> MLEQPYLDLAKKVLDEGHFKPDRTHTGTYSIFGHQMRFDLSKGFPLLTTKKVP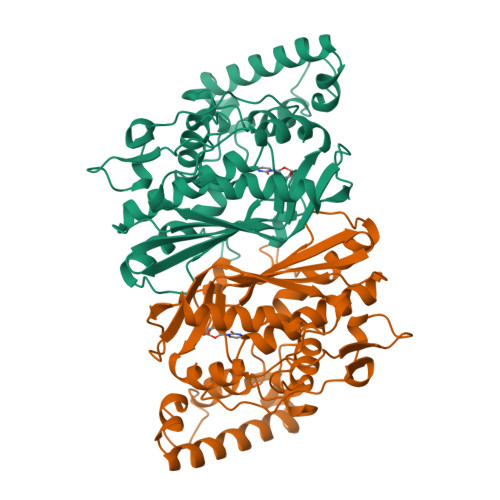FGLIKSELLWFLHGDTNIRFLLQHRNHIWDEWAFEKWVKSDEYHGPDMTDFGHRSQKDPEFAAVYHEEMAKFDDRVLHDDAFAAKYGDLGLVYGSQWRAWHTSKGDTIDQLGDVIEQIKTHPYSRELIVSAWNPEDVPTMALPPCHTLYQFYVNDGKLSLQLYQRSADIFLGVPFNIASYALLTHLVAHECGLEVGEFIHTFGDAHLYVNHLDQIKEQLSRTPRPAPTLQLNPDKHDIFDFDMKDIKLLNYDPYPAIKAPVAV> GKPLHEQLWYHGAIPRAEVAELLVHSGDFLVREGQSQPDYVLSVLWDGLPRHFIIQSLDNLYRLEGEGFPSIPLLIDHLLSTQQPLTK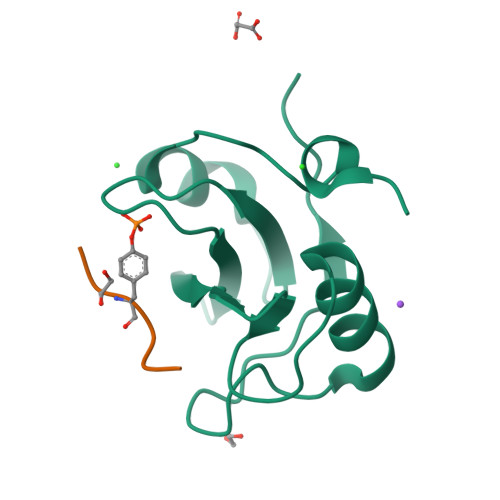KSGVVLHRAVPKSRA;> PPVYEPV>MVIPYVIEQTARGERVYDIYSRLLKDRIIFLGTPIDAQVANVVVAQLLFLDAQNPNQEIKLYINSPGGEVDAGLAIYDTMQFVRAPVSTIVIGMAASMAAVILAAGEKGRRYALPHAKVMIHQPWGGVRGTASDIAIQAQEILKAKKLLNEILAKHTGQPLEKV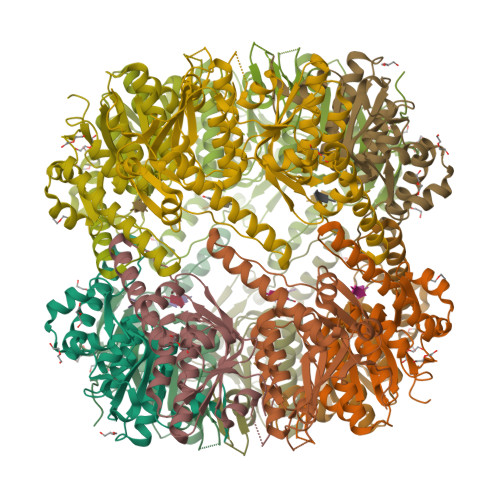EKDTDRDYYLSAQEALEYGLIDQVVTREEALEHHHHHHHH[7x]>[8x]MSLVKISNVRVRPLVLPLKQPYHWSYGIRESFAVNLIEIEADDGTVGIGECTVAPDQTGTAAILYRLAKHLVGHSPHDVAPLIARIFHQ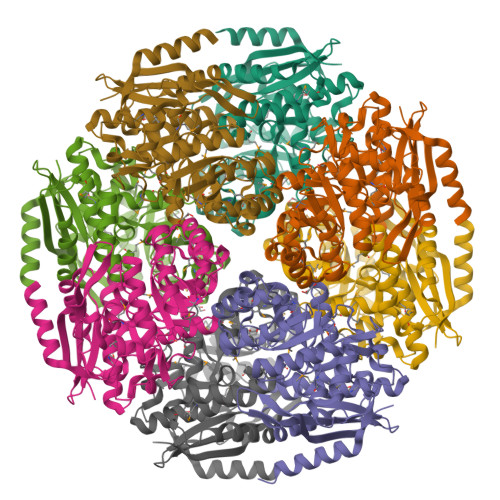EYLGHGANIMRAANQIFSGIDMAMWDLQGKLAGLPVHQLLGGAHRKAVGYFYFLQGETAEELARDAAVGHAQGERVFYLKVGRGEKLDLEITAAVRGEIGDARLRLDANEGWSVHDAINMCRKLEKYDIEFIEQPTVSWSIPAMAHVREKVGIPIVADQAAFTLYDVYEICRQRAADMICIGPREIGGIQPMMKAAAVAEAAGLKICIHSSFTTGITTCAEHHIGLAIPNLDDGNQIMWQLVQEDIVSSPDLTPKNGWLDAFRKPGLGFQLAEDLVAEGEGRYAASREGHHHHHH> SMLKLSAENESTPIQQLLEHFLRQLQRKDPHGFFAFPVTDAIAPGYSM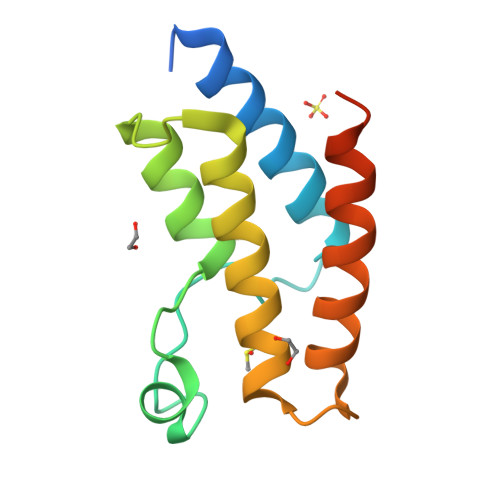IIKHPMDFGTMKDKIVANEYKSVTEFKADFKLMCDNAMTYNRPDTVYYKLAKKILHAGFKMMSKERLLALKRSMS> NLNS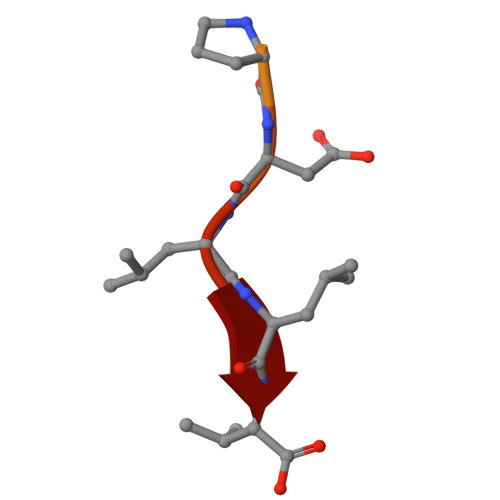SRVPDLLV> EQMSVETPSALADSSPHTAPGSAGRSLELGAADIQDLESFEAGRGALPARAYLQSDAPRLSLNGEWQFRLSPGSRVAPDDGWQLGEALNGFESLPVPSSWPMHGHGAPAYTNVQFPFAVEPPHVPEANPIGDHLVVFEAGPEFFPHALLRFDGIESAGTVWLNGVELGTTRGSRLAHEFDVSGILEQGENTLAVRVAQFSAASYVEDQDMWWLPGIFRDVTLQARPAAGIDDVFVHAGYDHITGEGILKVEASRGGQAIDAVVRVPELALELAAGTEVRVPAVEPWSAEVPKLYEAAVSAAGESVALQIGFRSIAIEDAQFKVNGRRILLRGVNRHEHHPRLGRVVPRDVVEAELRLMKQHNINAIRTSHYPPHPQFLALADQLGFYVVLECDLETHGFESAGWAQNPSDDPQWEDALVDRMRRTVERDKNHASVVMWSLGNEAGTGRNLAAMSRWTKDRDPSRPIHYEGDWSSEHVDVYSRMYASQAETALIGQGIEPALNDAALDARRRAMPFVLCQYVHAMGNGPGGMSEYQALFEKYPRLMGGFVWEWLEHGITVSTADGVDHYGYGGDFGEEVHDGNFVTDGLVDADRRPRPGLLDFKKVIEPLRIDVARDWT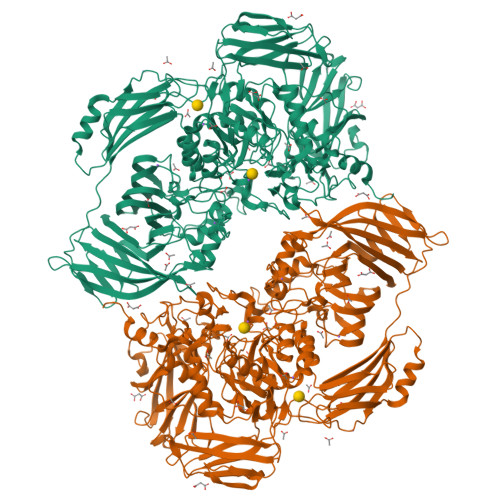GFTLRNGQDFADTSAFSFRYEVEADGGALDGGTVDVAPVAPQSETVVELPGSVAALAAGLSDGRPAVLTVRAVLGADSAWADAGHEVAWGQSVREPGAPVPPAPVEPVQVQDSELTLGPVVFSRATGMPTSIGGVPVEKLGLTLWWAPTDNDLGREWGGADERPLATQWKDAGLNRLHTRLLGISANPGQDGGETLTVRTRVSAADKQYGVLVDYTWSTDGETVGLRTQVRRDGTWVNRGFEVEWARIGLEFVLGEETELVSWFGQGPHQSYPDTGQGARAGWFSLPLAKMDVEYVRPQECGARSGSRSAALQLGGRTLEICGDPFALTVRPYSQDVLDAAAHRPDLKADGRTYLYVDHALRGVGTAACGPGVLEQYRLKPRDADFILTLKVRS>[8x]ISRLSTSPSTPPAPTAEDLARAQIPEQQRDQVASLMMVGVANYDQALDALNQGVGGIFIGSWTDENLLTEPGRNIEALREAVGRDFSVSIDFEGGRVQRATNILGDFPSPRVMAQTMTPE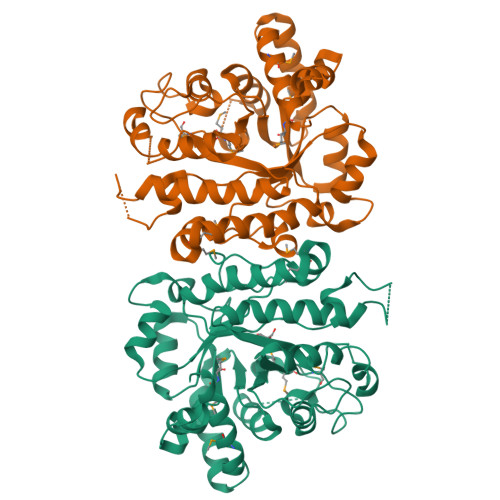QVEDLAEILGTGLAAHGVTVNFAPVVDVDAWGLPVVGDRSFSNDPAVAATYATAFAKGLSKVGITPVFKHFPGHGRASGDSHTQDVVTPALDELKTYDLIPYGQALSETDGAVMVGHMIVPGLGTDGVPSSIDPATYQLLRSGDYPGGVPFDGVIYTDDLSGMSAISATHSPAEAVLASLKAGADQALWIDYGSLGSAIDRVDAAVSSGEYPQEQMLASALRVQLLYI> MAKILCVLY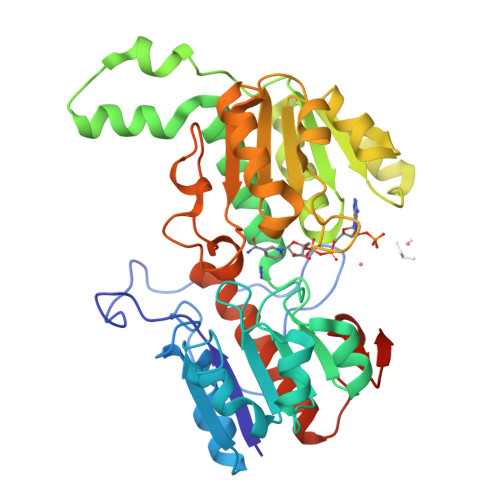DDPITGYPKSYARADVPKIDHYPGGQTAPTPKQIDFTPGELLGSVSGELGLRKYLEGLGHTLVVTSDKEGEDSVFERELPDAEIVISQPFWPAYLTPERIAKAKKLKLAVTAGIGSDHVDLEAAIKNGITVAEVTYSNSISVSEHVVMMILSLVRNYIPSYQWVIKGGWNIADCVERSYDLEAMHVGTVAAGRIGLAVLKRLKPFDVKLHYFSRHRLPESVENELGLTYHPSVEDMVKVCDVVTINAPLHPGTLDLFNDELISKMKRGAYLVNTARGKICNRDAVVRALESGQLAGYAGDVWFPQPAPKDHPWRTMPHHGMTPHISGTSLSAQARYAAGTREILECWFEERPIREEYLIVDGGKLAGTGAHSYTVSK>STRDYEIQRERIELGRCIGEGQFGDVHQGIYMSPENPAMAVAIKTCKNCTSDSVREKFLQEALTMRQFDHPHIVKLIGVITENPVWIIMELCTLGELRSFLQVRKFSLDLASLILYAYQLSTALAYLESKRFVHRDIAARNVLVSATDCVKLGDFGLSRYMEDSTYYKASKGKLPIKWMAPESINFRRFTSAS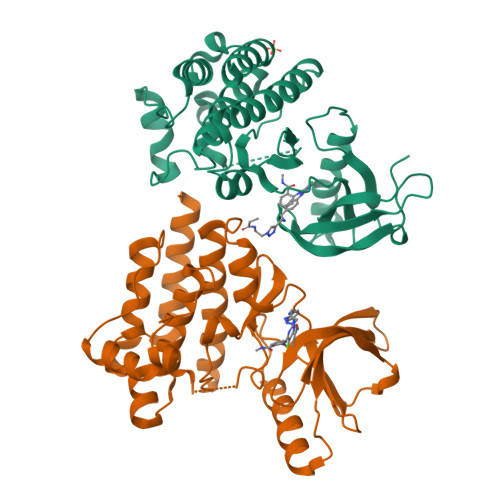DVWMFGVCMWEILMHGVKPFQGVKNNDVIGRIENGERLPMPPNCPPTLYSLMTKCWAYDPSRRPRFTELKAQLSTILEEEKLQ[2x]> MDETGKELVLVLYDYQEKSPRELTIKKGDILTLLNS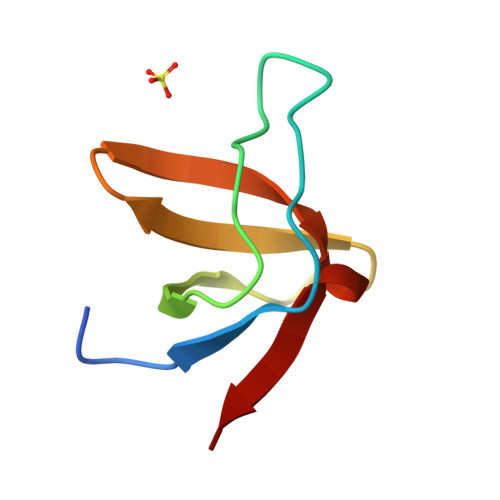TNKDWWKVEVNDRQGFIPAAYLKKLD>[4x]ME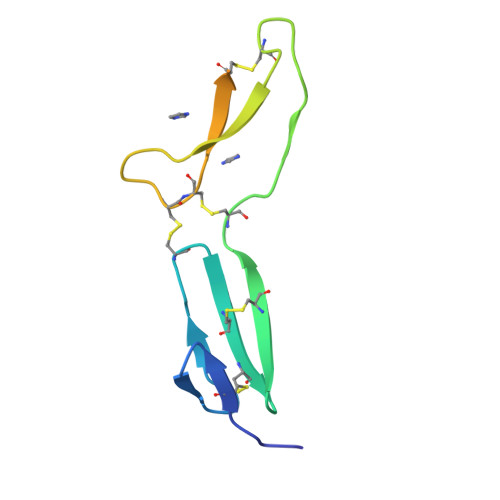GDNCVFDGVIYRNGEKFEPNCQYHCTCRDGQIGCVPRCQLDVLLPGPDCPAPKKVAVPGECCEKWTCGSEEKGTLGGLALPAYRPEATVGVELSD>[12x]MHWQTHTVFNQPIPLNNSNLYLSDGALCEAVTREGAGWDSDFLASIGQQLGTAESLELGRLANVNPPELLRYDAQGRRLDDVRFHPAWHLLMQALCTNRVHNLAWEEDARSGAFVARAARFMLHAQVEAGSLCPITMTFAATPLLLQMLPAPFQDWTTPLLSDRYDSHLLPGGQKRGLLIGMGMTEKQGGSDVMSNTTRAERLEDGSYRLVGHKWFFSVPQSDAHLVLAQTAGGLSCFFVPRFLPDGQRNAIRLERLKDKLGNRSNASCEVEFQDAIGWLLGLEGEGIRLILKMGGMTRFDCALGSHAMMRRAFSLAIYHAHQRHVFGNPLIQQPLMRHVLSRMALQLEGQTALLFRLARAWDRRADAKEALWARLFTPAAKFVICKRGMPFVAEAME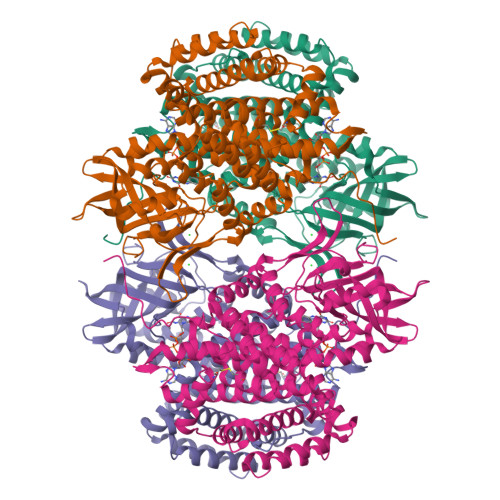VLGGIGYCEESELPRLYREMPVNSIWEGSGNIMCLDVLRVLNKQAGVYDLLSEAFVEVKGQDRYFDRAVRRLQQQLRKPAEELGREITHQLFLLGCGAQMLKYASPPMAQAWCQVMLDTRGGVRLSEQIQNDLLLRATGGVCV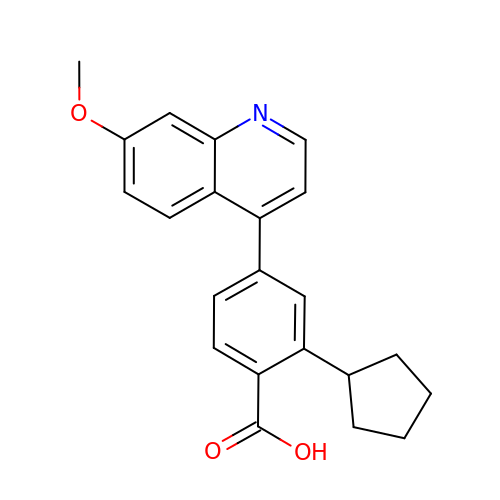2-cyclopentyl-4-(7-methoxyquinolin-4-yl)benzoic acid | C22 H21 N O3 | ISWSKRZAOHBEDP-UHFFFAOYSA-N> GMSKGEGTIANHLLEQQIKAFPKVAQQYYPRELSILRLQDAMKFVKELFTVCETVLSLNALSRSTGVPPELHVLLPQISSMMKRKIVQDDILKLLTIWSDAYVVELNSRGELTMNLPKRDNLTT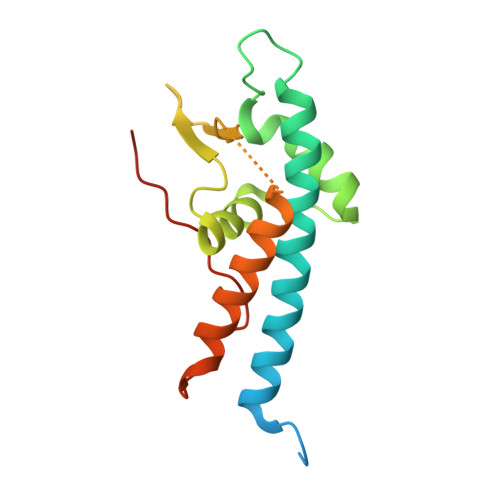LTNKSRTLAFVERAESWYQQVIASKDEIMTDVPAFKINKRRSSSN UNC-104/KIF1A was originally identified through genetic screens in C. elegans and is the primary kinesin motor for anterograde axonal transport of synaptic vesicle precursors. UNC-104/KIF1A belongs to the kinesin-3 subfamily, which can dimerize and can be found as an inactive monomer or a processive homodimer. The current model demonstrates that the activation of KIF1A involves the relief of its autoinhibition, a regulatory mechanism found in other kinesins. Previous studies showed that the motor domain of kinesin-3 family member KIF13B could interact with both NC and CC1 to form a compact self-folded monomer for autoinhibition.

As expected, in comparison to the autoinhibited wild type, both the T192Y and L397F mutations significantly restored the ATPase activity of the MD-NC-CC1 fragment, while the T408E mutation only moderately restored it. Because we could not obtain sufficient quantity and quality of UNC-104 protein for structural characterization, to further investigate the mechanism underlying the mutation-induced activation, we performed crystal screening of the three mutants of the KIF13B MD-NC-CC1 fragment. We successfully crystallized the T192Y-MD-NC-CC1 mutant and determined its structure by the molecular replacement method. The structure was refined to 2.3 Å with Rwork/Rfree of 18.2%/24.1%. In the structure of the T192Y-MD-NC-CC1 mutant, we could trace the electron densities of the motor domain (with bound ADP-Mg2+) and NC, but not of CC1, possibly due to the intrinsic flexibility of CC1 upon dissociation from the motor domain. Although only one molecule was found in the asymmetric unit of the crystal, a MD-NC dimer could be formed by a crystallographic two-fold symmetry axis. This demonstrates that the T192Y-MD-NC-CC1 mutant can indeed adopt an active dimeric conformation, mediated by the NC coiled-coil. Upon superimposition, the structure of the T192Y-MD-NC-CC1 mutant was very similar to that of the active MD-NC dimer, which also supports the notion that this is the active conformation of the T192Y-MD-NC-CC1 mutant. In the autoinhibited conformation of the wild type MD-NC-CC1, T192 sits in the interaction interface between the motor domain and CC1b, while in the T192Y-MD-NC-CC1 mutant, the bulky aromatic sidechain of Y192 protrudes from the motor domain. The T192Y mutation is therefore likely to introduce a steric hindrance that could prevent CC1b from interacting with the motor domain, which would ultimately activate the motor for processive movement.

> MGDSKVKVAVRVRPMNRREIDLHTKCVVDVEANKVILNPINTNLSKGDARGQPKIFAYDHCFWSMDESVREKYAGQDDVFKCLGENILQNAFDGYNACIFAYGQTGSGKSYTMMGTADQPGLIPRLCSGLFERTQKEENEEQSFKVEVSYMEIYNEKVRDLLDPKGSRQTLKVREHSVLGPYVDGLSKLAVYSYKDIESLMSEGNKSRTVAATNMNEESSRSHAVFKITLTHTLYDVKSGTSGEKVGKLSLVDLAGSERATKTGAAGDRLKEGSNINKSLTTLGLVISALADQGAGKNKNKFVPYRDSVLTWLLKDSLGGNSKTAMVATVSPAADNYDETLSTLRYADRAKHIINHAVVNEDPNARIIRDLREEVEKLREQLTKAEAMKSPELKDRLEESEKLIQEMTVTWEEKLRKTEEIAQERQKQLESHHHHHH> MADAGKREGRVFAPYS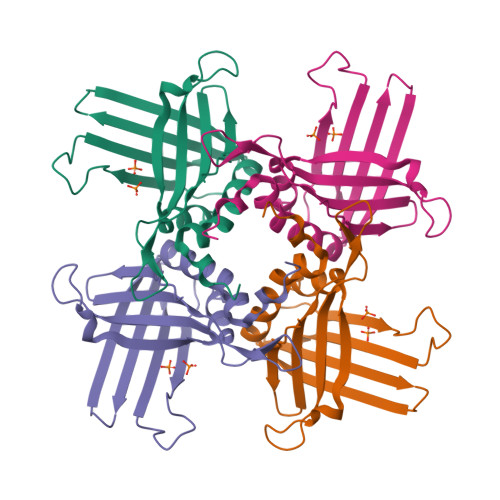VFKGKAALSAEPRLPTFNRLDSGGVKLNRRGVIMLTFWPSVGERKYDWEKRQLFALSATEVGSLISMGTRDSSEFFHDPSMLSSNAGQVRKSLSIKPNADGSGYFISLSVVNNNLKTNDRFTVPVTTAEFAVMRTAFSFALPHIMGWDRFTNRPLEHHHHHH> YGPHADSPVLMVYGLDQSKMNCDRVFNVFCLYGNVEKVKFMKSKPGAAMVEMADGYAVDRAITHLNNNFMFGQKMNVCVSKQPAIMPGQSYGLEDGSCSYKDFSESRNNRFSTPEQAAKNRIQHPSNVLHFFNAPLEVTEENFFEICDELGVKRPTSVKVFSGKSERSSSGLLEWDSKSDALETLGFLNHYQMKNPNG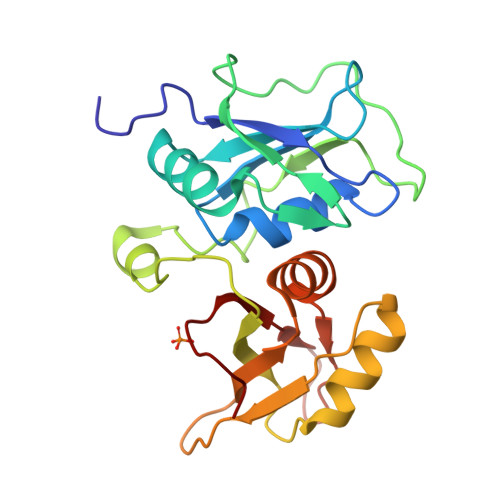PYPYTLKLCFSTAQHAS Here, we report on the structure and reactivity of such a deviant enzyme, termed CooS‐VCh. Its structure reveals the typical CODH scaffold, but contains an iron‐sulfur‐oxo hybrid‐cluster. Although closely related to true CODHs, CooS‐VCh catalyzes neither CO oxidation, nor CO2 reduction. The active site of CooS‐VCh undergoes a redox‐dependent restructuring between a reduced [4Fe‐3S]‐cluster and an oxidized [4Fe‐2S‐S*‐2O‐2(H2O)]‐cluster.

While the [2Fe‐2S] subsite with Fe2 and Fe3 coordinated by Cys338 and Cys480 hardly changes upon reduction, the two μ2‐oxo atoms and the water molecule disappeared, resulting in a [4Fe‐3S]‐cluster. The S3 atom, before part of a cysteine persulfide, is now embedded in the cluster after a shift of 3.1 Å, becoming a μ3‐ligand for Fe2, Fe3 and Fe4. Fe4, coordinated in the oxidized state by two oxo‐bridges, a sulfur and a water molecule, now relocates to an exo position by a 2.1 Å movement and is coordinated by His259, Glu295 and S3 and Sγ‐Cys521, for which Cys521 undergoes a 120° rotation to complete the tetrahedral coordination of Fe4. Fe1 loses its water ligand upon reduction and adopts a trigonal‐planar coordination with open coordination sites in the reduced state. When the hybrid‐cluster is reduced, it rearranges so that the persulfido sulfur becomes a μ3‐bridging ligand within the cluster. This switch of position for S3 and Sγ‐Cys521 opens the channel, providing access to the hybrid‐cluster cavity (open conformation in Figure 7B).

>[2x]MATKTSIHPSVNELYQRLAEDQLSNCFDRFDPQEKIRCNYCELGVSCQLCSNGPCRINEKVGATLGVCGINADGMAMRYMLLRNVMGTSTYTYHAYEAYKTLKMTALGNTPFTITDKDKLYQMAKDLELNTEGKPEDVAVRLSDFLIWELYRDYDEPGKMIEVYAPLKRKEVWRKLGIYPAGPLHELKDAAASCLTNVDGDYVSLATKGLRLGLSCIYGAQIGLELVQDILFGTGMPHEMDVDLGIFDADYINIVFNGHEPFVGVALILAAKEAVNQDKAKAAGAKSLRIYGSIESGQEVVQRFQKDEVFRGLTGNWLTIEPMLATGAVDVLAMDMNCSPPNLGPLAEKYGATLVSVSRLVRFPGIHHFLDYKPSEVREIAQKIIDIAVDSFKNKRHGKITPKIPANIQKAITGFTPEAILKALGGSINPLIEVIKAGKIKGAVGLINCTTLKNGPQDYVTVNLAKELIKRDILILSGGCGNHALEVAGLCNLDAINLAGPGLSEVCRNLNIPPVLSFGTCTDTGRISLVVTALANALNVDTADLPVAVTAPMYMEQKATIDALFALAYGLYTHVAPDPPVMGAPNLVKLLTRDLPSITGGRIAVGSDPVKVADDILAHINDRRAKLGI> GSLPEVLQAPVGSSILVQCHYRLQDVKAQKVWCRFLPEGCQPLVSSAVDRRAPAGRRTFLTDLGGGLLQVEMVTLQEEDAGEYGCMVDGAR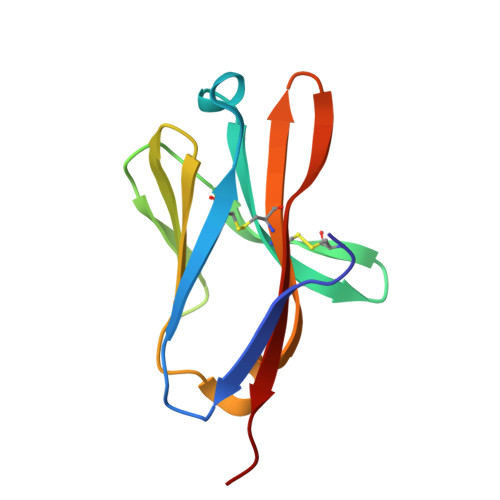GPQILHRVSLNILPP>MAKDKEF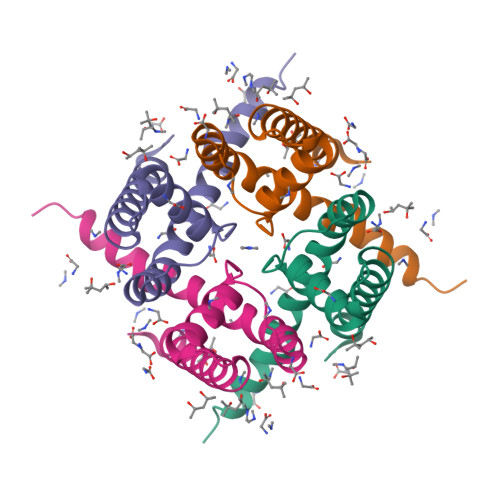QVLFVLTILTLISGTIFYSTVEGLRPIDALYFSVVTLTTVGETPPPQTDFGKIFTILYIFIGIGLVFGFIHKLAVNVQLPSILSNLVPR[4x]>MAMPRHGRRPARCSSNRASQWLLLVLGVALAASPRFLLLVEAATYTLTLDKLGPTVNPTTSDAVTFTATVASPDSTTAVFFTLDYGDGVTAETTRTTTGALSTTPTANLVSAGTYTVTYASIGTKFVTLRLYDSAVAPGVLLASKTVPIYVEDSTLTATLLQSGVPRLNLAFSGFKGRVSSSTANRADMWATIQLDTAPGVFESSRIFIGIAPTASTNYDFVIPDQVYNLEGAKTTVLRIYDAPVGGTLLRTFTPAAANAVYVVDPSKYVLTLTVGPTSVTTADQVTFTQTTTEVSYSASATSPILQWRFNWDDPSVVETPLAYPDALTAASNFPTTATAVSSAAASTFRYTSTGSKNARLRLYDGANNVIAEKIVVITVSNAGYTLALAKTTADPVTTDDTIAFSAGAKHLSSTSQVWWTIDYGAGESSPRTALTMTNVGAAAPNAIASLSNQYTSGGTKLATLRIYDRDGVGANTGLLLASTTVTFTVTPVLYALESAVEPFSPIATVAAKWSFRIQRSKATPAGVTESIKCAFFGADTGTAPADLAAWLTAANGAGGLTATILPSSIPSDIISFTRTYAAAAASLQGKLQCFIGSTPLWDPYYPTPVFQVLAAAPTYTLSASVTPAVVPVDTATLWTYNIIRSVPVPAGGPSLPILCSFWDGKTGAAPTTDAGWAALAGSANGKGTSMAPGSTTATCSFTPSYSTTGTATPTLQLIQNSFALDAATTVGFLSPVYTAPAFATVTAASYTISSYLNPVTPVAGGAAAVWRIVITRNAAVTASAKTLTCQMPDNGQGGSPADVTADIAVGGTTTVCVFSIAGYTTATPGPYFATVNVVDGAVTTSHITKNFTVLASGTTAPTYAVTSVVSPATPVKVSTPVTYTFTITRTTAVPAGGIPQPIICEFFNGEGTAPASAAAYWRVSTTIPDADTVVAVMAPGETTTTCTFTTYYTTVSAGGFTAKLMVFGESATAAPLLTSLSVTPSQLLAAVHSFATPMVVAAAVVAVESTTISPNYNPTTPYTNIPTYFTFTLLRDPPVPPSASSGVQFACALYTGQNVNPASAPSAITDAVYKTFTDVTTAVATDANYFADQQLRVVTMAPGTGRVSCTFPTLYAAAGPFSPKFFVFEYASSTVGANALAVADTVTSLTSFTTQAAPTFITGPTNVPQRVPLPKGFRTTCFDGYELIFSNDNYTNGVRVAVDAYPYPVGQCRKCPGGTATMDGYRCIPCPSGYWSNEGARECTACPAGTIAKPAALTARAKYSIDPTTYHFVTHLAMGPESCKKCPKGYFQPNIAGTVCLPCPSGFVSTSGATGCTACSEGTYHTDGVGTTTPGEATSLDTTDTFGSIYPIIPNTCRQCPANTYLPLRGQAAIASMNLAAVSSATPCRPCEDGTWSKAGAAGCQKCPPGTYRNTWFSGQLGSPFITADGVPVATTLTELGSGCSQCPPGTYAPTFGMSVCLPCPAGTFASAPGATACQQCKPGTNSLMGDRTQQMALVVTNAANDFPALRAYTISGMVAGPAYAKPIVTGPDTNFFMAGKSETCSTNLPGYYTDVDGLPIQLPCKPGTFMPFDTATANLLDTGLTVDGTQCYTCQTGTFNDEFSQPVCKACWSGSFASKRGLPTCEIAQPGTFTNVAAAANATFNTATLIPTGLVKGAQAPTPCGMGYFQSSAETTTCTACAVGTYADQAGLAACKPCQPGRYQNSIGQRVCKPCDMGTYSRYGGELCTKCPAGTVASKTGSSQCTPCAAGFYANAP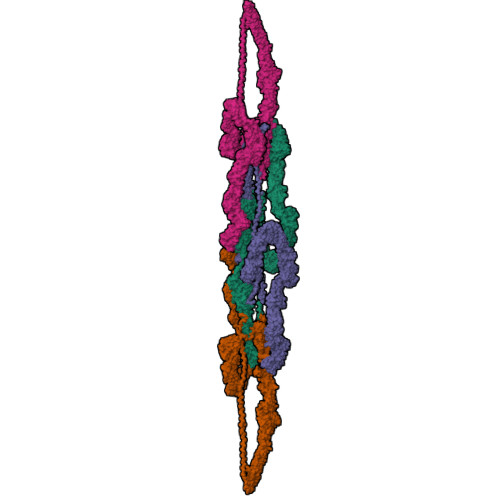DSATSCRACPRGYYGPYSGAYADNLGDEFEGPRGCYKCPYDFFADRPGVRQCTACPPLDLGGGNLVEQCTEDLGSQRCKPCSLLSKPKTARTEQSPPPPSPSPPPPPPPSPRPPSPNPPSPRPPSPAPPSPNPPPTSPPPSPPPSPPPPRPPPPPPPPPSPPPPNRSPPPPPPASSAINPGGGVNQNGDPVGHRRAILSLMEDEDAEAAQEEQAIVDVDAEMQPQDDE[4x]> MASPDSATLREPVVLPPMPGEHEARAAYPPIGLERSRVTGGRLVFDRDEGFDRALAQGFFLVRIPEGTDPAAGDRFAAHFHEERAGGDPLDAYRGYRHVRVPGDYQGYFDREHDQWENFYVERDNWDVLPSEVARVGRGMAGLGVTILRGVLEHLRLPREHWARVTGGLTEDRGHQMLAFNHFRSHKGVRGSKFHRDSGWVTVLRSVDPGLLALVDGRLWAVDPEPGHFIVNFGSSLEVLTERLDRPVRANVHGVVSTERAPGQPDRTSYVTFLDSDLTGTVYRFENGTPRPLQSVAEFAGQEVGRAYDDSGALEHHHHHHHH

Here we report the mechanism of three Fe(II)/α-ketoglutarate-dependent dioxygenases in bicyclomycin synthesis, which depicts the natural tactic to sequentially hydroxylate specific C−H bonds of similar substrates (cyclodipeptides). Three αKGDs (BcmE/BcmC/BcmG) catalyze site- and stereo-selective hydroxylation of inert C−H bonds in BCM’s (bicyclomycin) cyclic dipeptide scaffold (Fig. 1b3), one of the simplest peptide derivatives without additional functional groups. Our hypothesis posits distinct regulatory mechanisms: BcmE employs steric hindrance, BcmC relies on inherent reactivity, while BcmG utilizes a directing group to control C–H hydroxylation. Although these three enzymes share only 35–42% amino acid identities, the overall structures are similar, and r.m.s.d. values are 0.70 Å (SsBcmE vs SsBcmC), 1.07 Å (SsBcmE vs PaBcmG) and 0.87 Å (SsBcmC vs PaBcmG), respectively.

The carbonyl group of the amide part of the DKP ring is stabilized by a π-π stacking interactions with the aromatic ring F273. Additionally, Y308 forms hydrogen bonds with the NH group of the DKP ring and the hydroxyl group of Y120. Two water molecules mediate the hydrogen interactions between carbonyl groups of DKP and residues R111 and D275. The 5-methyl group of the DKP ring is oriented towards the iron center, suggesting that hydrogen abstraction is likely to occur preferentially at the C-5a position. This observation is consistent with the activity of SsBcmET307A. The presence of a rotatable single bond between C-4 and C-5 brings the possibility of C-7 closer to the iron center, thereby preserving the reactivity observed in the wild-type SsBcmE. Given that the mutant complex structure did not fully exhibit the characteristics of the wild-type protein complex, we modeled the structure of wild-type SsBcmE based on the mutant quaternary complex structure and docked substrate 1 to the active sites. We found the steric hindrance of T307 could bring C-7 closer to the iron center. Conversely, mutations Y120F, V304T, T307A, and Y308F enhanced total activities (72%–95% total conversion yields) and produced a new C-5a-hydroxylated product 1a (2%–27% conversion yields). As expected, the dominant active conformations for hydroxylation in the F273A, T307L and T307A systems are C-6, C-2’ and C-5a (shown in the dotted rectangle: 49/5000, 90/5000 and 14/5000), respectively, which is consistent with our mutagenesis results and structures, particularly the crystal structure of SsBcmET307A•FeII•αKG•1.>[2x]MNNFGNEEFDCHFLDEGFTAKDILDQKINEVSSSDDKDAFYVADLGDILKKHLRWLKALPRVTPFYAVKCNDSKAIVKTLAATGTGFDCASKTEIQLVQSLGVPPERIIYANPCKQVSQIKYAANNGVQMMTFDSEVELMKVARAHPKAKLVLRIATDDSKAVCRLSVKFGATLRTSRLLLERAKELNIDVVGVSFHVGSGCTDPETFV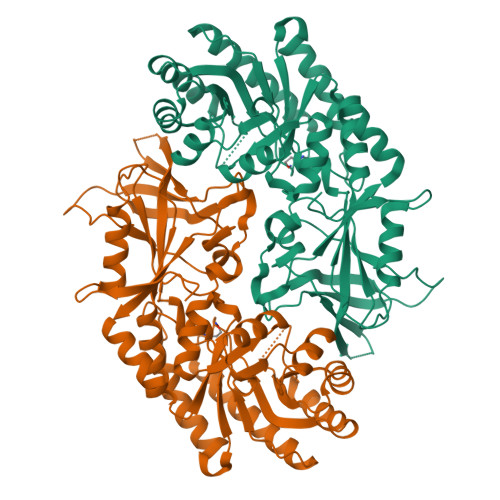QAISDARCVFDMGAEVGFSMYLLDIGGGFPGSEDVKLKFEEITGVINPALDKYFPSDSGVRIIAEPGRYYVASAFTLAVNIIAKKIVLKEQTGSDDEDESSEQTFMYYVNDGVYGSFNCILYDHAHVKPLLQKRPKPDEKYYSSSIWGPTCDGLDRIVERCDLPEMHVGDWMLFENMGAYTVAAASTFNGFQRPTIYYVMSGPAWQLMQQFQNPDFPPEVEEQDASTLPVSCAWESGMKRHRAACASASINV>DNFEEYAQLEEYASAEDISRVRAELLTCPELNTSLAGTIIEIDKNYAKSILITTSEMVADDQGLIFDAFIFAAANYVAQASINKEFSVII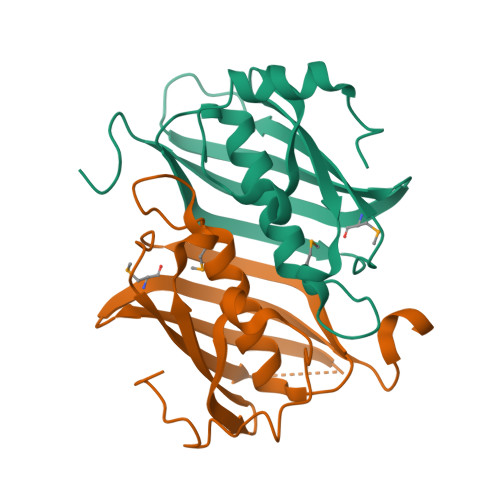GSKCFFYAPLKLGDVLELEAHALFDETSKKRDVKVVGHVKEIKMFEGTIQVVSTDEHIFKLK[8x]>SAKECRCQCIKTYSKPFHPKFIKELRVIESGPCCANTE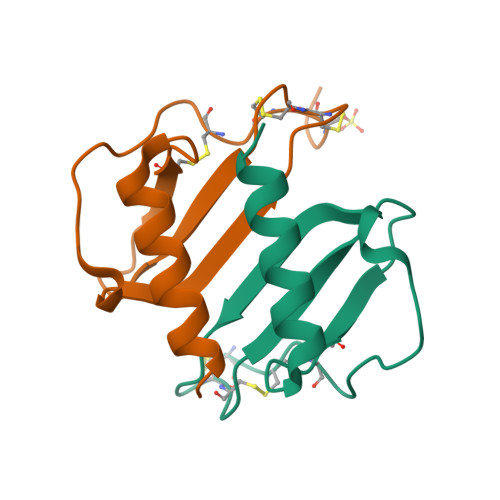IIVKLSDGRELCLDPKENWVQRVVEKFLKRAENS[4x]>[4x]MVHYKLTYFAIRGAGECARQIFALADQEFEDV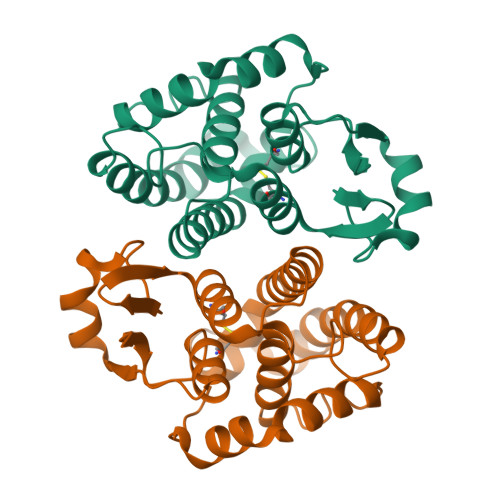RLDKEQFAKVKPDLPFGQVPVLEVDGKQLAQSLAICRYLARQFGFAGKSTFDEAVVDSLADQYSDYRVEIKSFFYTVIGMREGDVEQLKKEVLLPARDKFFGFITKFLKKSPSGFLVGDSLTWVDLLVSEHNATMLTFVPEFLEGYPEVKEHMEKIRAIPKLKKWIETRPETLF>MAHHHHHHMEIRDNVFLITGGASGLGAGTARLLTEAGGKVVLADLNQDAGE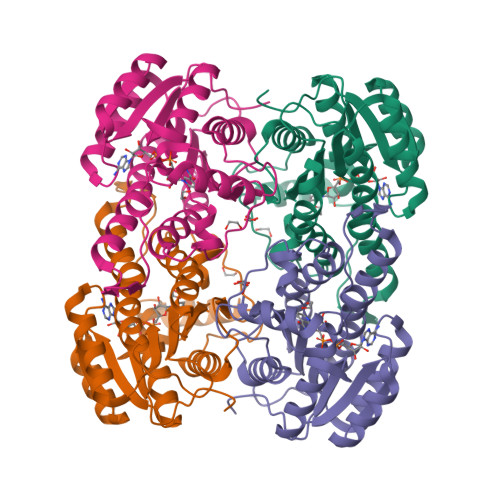ALARELGGVFVRCDVAREEDAQAAVAAATKLGTLRGLVNCAGIAPAAKTVGKDGPHPLELFAKTITVNLIGTFNMIRVAAAAMAANEPAPTGERGVIVSTASVAAFDGQIGQAAYAASKAGVAGMTLPIARDLSRNAIRVMTIAPGIFETPMLLGMPQEVQDALGAMVPFPPRLGKPAEYAMLVRQIFENPMLNGEVIRLDGAIRMQPK[8x]> MSAEKLFTPLKVGAVTAPNRVFMAPLTRLRSIEPGDIPTPLMGEYYRQRASAGLIISEATQISAQAKGYAGAPGLHSPEQIAAWKKITAGVHAEDGRIAVQLWHTGRISHSSIQPGGQAPVSASALNANTRTSLRDENGNAIRVDTTTPRALELDEIPGIVNDFRQAVANAREAGFDLVELHSANGYLLHQFLSPSSNQRTDQYGGSVENRARLVLEVVDAVCNEWSADRIGIRVSPIGTFQNVDNGPNEEADAL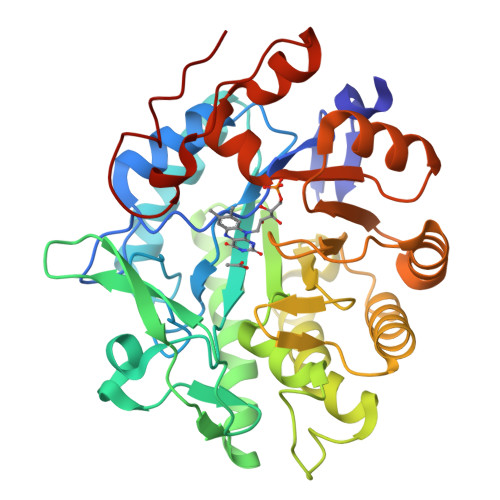YLIEELAKRGIAYLHMSETDLAGGKPYSEAFRQKVRERFHGVIIGAGAYTAEKAEDLIGKGLIDAVAFGRDYIANPDLVARLQKKAELNPQRPESFYGGGAEGYTDYPSL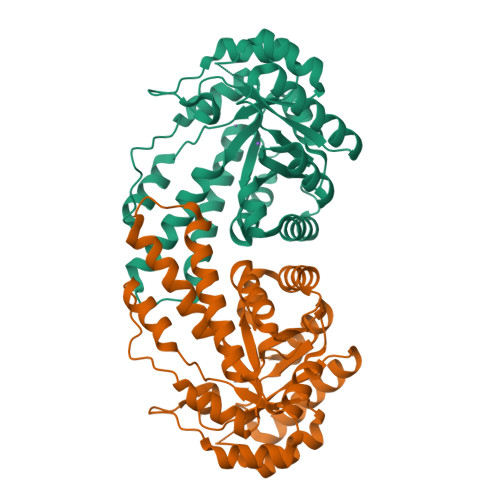>[2x]MLVKGNEILLKAHKEGYGVGAFNFVNFEMLNAIFEAGNEENSPLFIQASEGAIKYMGIDMAVGMVKIMCERYPHIPVALHLDHGTTFESCEKAVKAGFTSVMIDASHHAFEENLELTSKVVKMAHNAGVSVEAELGRLMGIEDNISVDAKDAVLVNPKEAEQFVKESQVDYLAPAIGTSHGAFKFKGEPKLDFERLQEVKRLTNIPLVLHGASAIPDNVRKSYLDAGGDLKGSKGVPFEFLQESVKGGINKVNTDTDLRIAFIAEVRKVANEDKSQFDLRKFFSPAQLALKNVVKERMKLLGSANKI> KEVCYTPLGCFSDDKPWAGTLQRPLKSLPWSPEEVNTRFLLYTNKNPDSYQLITARDVATIKSSNFQSSRKTHFVIHGFRDRGEDSWPSDMCKKILQVETTNCISVDWSSGAKAEYTQAVQNIRIVGAETAYLIQQLLTELSYNPENVHIIGHSLGAHTAGEAGRRLEGRVGRVTGLDPAEPCFQDASEEVRLDPSDAQFVDVIHTDASPMLPSLGFGMSQKVGHMDFFPNGGKQMPGCKRSSFSTFIDINGIWQGAQDYLACNHLKSFEYYSSSILNPDGFLAYPCDSYDKFQENGCFPCPAGGCPKMGHYADQYKEK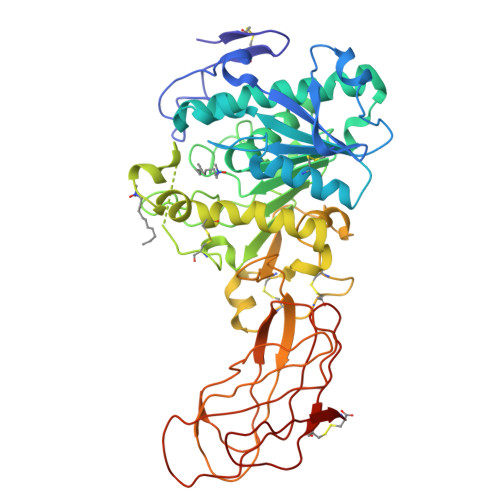TSAVEQTFFLNTGESGDYTSWRYRVSITLAGSGKANGYLKVTLRGSNGNSKQYEIFKGSLQPDSSYTLDVDVNFIIGKIQEVKFVWNKTVLNLSKPQLGASRITVQSGADGTEYKFCGSGTVQDNVEQSLYPC>GSLLRQELSCPLCLQLFDAPVTAECGHSFCRACLIRVAGEPAADGTVACPSCQAPTRPQALSTNLQLSRLVEGLAQVPQGHCEEHLDPLSIYCEQDRTLVCGVCASLGSHRGHRLLPAAEAQARLKTQLPQQKMQLQEASMRKEKTVAVLEHQLVEVEETVRQFRGAVGEQLGKMRMFLAALESSLDREAERVRGDAGVALRRELSSLNSYLEQLRQMEKVLEEVADKPQTEFLMKFSLVTSRLQKILSESPPPARLDIQLPVISDDFKFQVWKHMFRHLMPALEELTFDPSSAHPSLVVSSSGRRVECSDQKAPPAGEDTRQFDKAVAVVAQQLLSQGEHYWEVEVGDKPRWALGVMAADASRRGRLHAVPSQGLWLLGLRDGKILEAHVEAKEPRALRTPERPPARIGLYLSFADGVLAFYDASNPDVLTPIFSFHERLPGPVYPIFDVCWHDKGKNAQPLLLV[4x]

Tripartite motif-containing protein (TRIM)72 (mitsugumin 53; MG53) has been determined to rapidly nucleate vesicles at the site of membrane damage, but the underlying molecular mechanisms remain poorly understood. Here we present the structure of Mus musculus TRIM72, a complete model of a TRIM E3 ubiquitin ligase. TRIM72 is a member of the class IV TRIM proteins, which is the largest subtype among the 11 groups of TRIM proteins. Its domain organization includes an RBCC domain followed by a PRY motif associated with a SPRY domain identified in splA kinase and ryanodine receptors (PRYSPRY) domain.

After introducing point mutations and deletions, we were finally able to resolve molecular models of mouse TRIM72, including RING-deleted (ΔRING, 2.75 Å; the highest resolution is in parentheses), full-length (FL, 4.6 Å) and wild-type (WT, 7.1 Å) TRIM72. At the N terminus, a catalytic RING exists in a bent conformation near the other protomer of the CCD. In our crystal structures of TRIM72, the key residue Gln57 in the RING domain was observed near Arg207′ in the CCD through the bent RING conformation. We also observed that the electron density map of the RING domain appears in only one of the four crystal structures of TRIM72 FL, suggesting that the RING domain is intrinsically flexible. Based on the experimental SAXS profiles, the calculated models showed that the RING domain is highly dynamic and does not prefer the bent conformation. Additionally, an AlphaFold58 prediction suggested that TRIM72 has the extended conformation of the RING domain, similar to one of the models calculated by SREFLEX. Therefore, we conclude that the RING domain is highly flexible in both the TRIM72 dimer and oligomer on the phospholipid membrane. Next to the RING domain, the B-box domains are located at each end of the CCDs and contact the H1 and H2′ helices of the CCDs in a hydrophobic manner.>[10x]NKGSIEGREPAVYFKEQFLDGDGWTSRWIESKHKSDFGKFVLSSGKFYGDEEKDKGLQTSQKARFYALSASFEPFSNKGQTLVVQFTVKHEQNIDCGGGYVKLFPN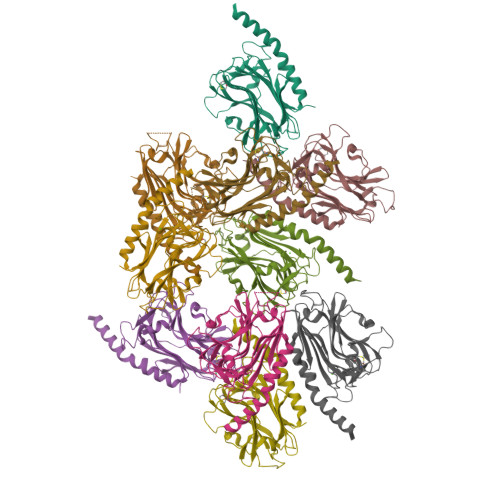SLDQTDMHGDSEYNIMFGPDICGPGTKKVHVIFNYKGKNVLINKDIRCKDDEFTHLYTLIVRPDNTYEVKIDNSQVESGSLEDDWDFLPGSGDPSIYAYDNFGVLGLDLWQVKSGTIFDNFLITNDEAYAEEFGNETWGVTKAAEKQMKDKQDEEQRLK> GSHMTSSANEDMPVERILEAELAVEPKTETYVEANMGLNPSSPNDPVTNICQAADKQLFTLVEWAKRIPHFSELPLDDQVILLRAGWNELLIASFSHRSIAVKDGILLATGLHVHRNSAHSAGVGAIFDRVLTELVSKMRDMQMDKTEL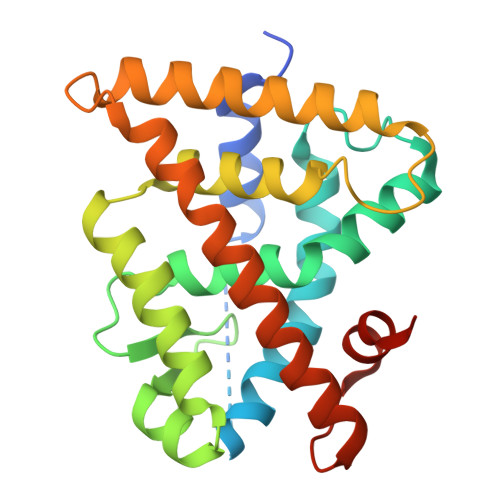GCLRAIVLFNPDSKGLSNPAEVEALREKVYASLEAYCKHKYPEQPGRFAKLLLRLPALRSIGLKCLEHLFFFKLIGDTPIDTFLMEMLEAPHQMT> MLSKALQRGIARAFSTTAKKEAPKTVKANGQVSQVIGAVVDVQFEGELPQILNALEVQGTQHRLVLEVAQHLGDSRVRTIAMDSTEGLVRGQPVVDTGLPISVPVGPGTLGRIMNVIGEPIDQRGPIKAAKLYPIHRDAPSFTDQATSAEILVTGIKVVDLLAPYARGGKIGLFGGAGVGKTVLIQELINNVAKHHGGYSVFAGVGERTREGNDLYHEMMDSKVISVKEGESRCALIFGQMNEPPGARARVGLTGLTVAEYFRDEEGKDVLLFVDNIFRFTQACSEVSALLGRIPSAVGYQPTLATDLGALQERITTTQKGSITSVQAIYVPADDLTDPAPATTFAHLDATTVLNRGLTELGIYPAVDPLDSTSRMLDPITIGEEHYTVARGVQKLLQDYKSLQDIIAILGVDDLSEEDKLVVARARKVQKFLSQPFFM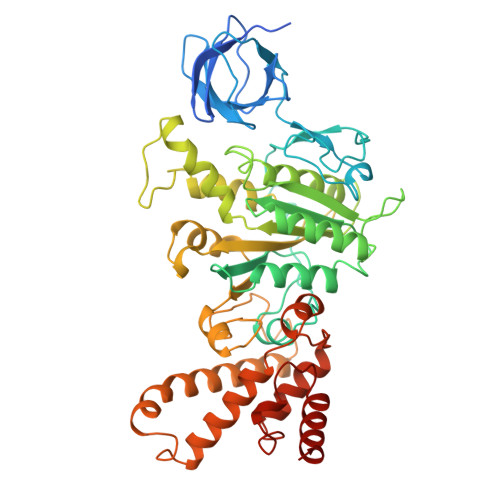SEVFSGIPGRFVNLKQNIASFKALLEGAGDEYPESCFYMKGDLEESLAAGRADALKSK Mupirocin, a clinically used natural antibiotic, inhibits isoleucyl-tRNA synthetase (IleRS), an enzyme that links isoleucine to its tRNAIle for protein synthesis. Two IleRSs, mupirocin-sensitive IleRS1 and resistant IleRS2, coexist in bacteria. Specifically, type 1 proteins (IleRS1) are strongly inhibited by mupirocin (Ki in low nanomolar range), while IleRS2, which are homologous to IleRSs from the eukaryote cytosol, exhibit resistance to mupirocin concentrations that are about three orders of magnitude higher. AARSs catalyze the formation of AA-tRNA in two steps within the same active site. The amino acid is first activated by ATP to form an aminoacyl-adenylate (AA-AMP) intermediate, followed by the transfer of the aminoacyl moiety to the tRNA.

To test this, we exchanged the natural HXGH motif in IleRS1 from P. megaterium and Escherichia coli with GXHH. GXHH-mutants showed a lack of product formation during prolonged reaction times even at 15 µM enzyme, confirming that the active site of IleRS1 cannot productively accommodate the non-canonical motif. Apart from wild-type PmIleRS1 and PmIleRS2, both of which harbor the canonical HXGH motif, we also structurally characterized their corresponding GXHH mutants, all in complex with a non-hydrolyzable analog of the isoleucyl-adenylate reaction intermediate, Ile-AMS. At the level of the overall fold, the WT enzymes and corresponding GXHH mutants are highly superimposable. However, while the binding of Ile-AMS to the active sites of both GXHH mutants parallels its binding to the corresponding wild-type enzymes, some distinctions that are mainly related to the precise accommodation of the adenine base emerged. In PmIleRS1, introducing the GMHH mutation leads to a 1.5 Å shift of the adenine base and a 2.1 Å move of Phe586, which loses its stacking with the adenine moiety. Such a distorted geometry of the active site likely results in a non-productive binding of the ATP substrate and concomitant loss of mut-GMHH-IleRS1 activity. In PmIleRS1, where no rearrangement of either HXGH or GXHH motif has been observed, the histidine at the third position promotes mispositioning of the adenine moiety, resulting in the abolished activity of mut-GVHH-PmIleRS1.

> MEYKDTLLMPKTEFPMRGNLPNREPKMQEQWAEMNIYEKVQKRTEGRPLFVLHDGPPYANGDIGMHHALNKILKDFIVRYKSMSGFCAPYVPGWDTHGLPIETALTKNKKVNRKEMTVAEFRKLCEQYAWEQVNGQREQFKRLGVRGDWDNPYVTLQPQYEAQQIKVFGDMAKKGYIYKGLKPVYWSPSSESALAEAEIEYYDKRSASIYVAFNVKDGKGVLEQDEKFIIWTTTPWTMPANQGIAVNPELQYSVVEADGAKYVVATELIETVAKEIEWADYKTLRTVKGSELERVVAEHPIYKRDSLVVLGDHVTTDAGTGCVHTAPGHGEDDFIVGQKYGLEVLCPVDSKGHMTNEAPGFEGLFYDKANKPITDKLEEEGALLKLSFITHSYPHDWRTKKPTIFRATAQWFASIKDFREDLLKAVEKTKWVPTWGETRLYNMVRDRGDWCISRQRAWGVPIPVFYAENEEPIITDETIEHVSNLFREHGSNVWFEREAKDLLPEGFTHEGSPNGRFTKETDIMDVWFDSGSSHQAVLEEREDLQRPADLYLEGSDQYRGWFNSSLSTSVAVTGEAPYKGVLSHGFALDGEGRKMSKSLGNVVIPEKVMKQLGADILRLWVASVDYQADVRVSDNILKQVAEVYRKIRNTFRFLLGNLADFNPTTDAVAVEDLREVDRYMLVKLNKLIDKVKKSYDSYEFSSIYHAVHNFCTIDMSSFYLDFAKDVLYIEAENNVERRSIQTVLYETLLSLTKLVSPILSHTADEVWVHIPNVTEESVQLVDMPEVQEIEGADQLVEKWDAFMELRDEVLKALEQARNEKVIGKSLEAKLTLYPTADTKELLASISENVGQLFIVSDLEVAEGEAPAEAQKFSYASIVVSKAEGEKCERCWVVSPTVGEDQDHPTLCTRCADVVKNHYVQQ> KEKTGQVKHKNQATHKEFSQLEKKFDARLGVYAIDTGTNQTIAYRPNE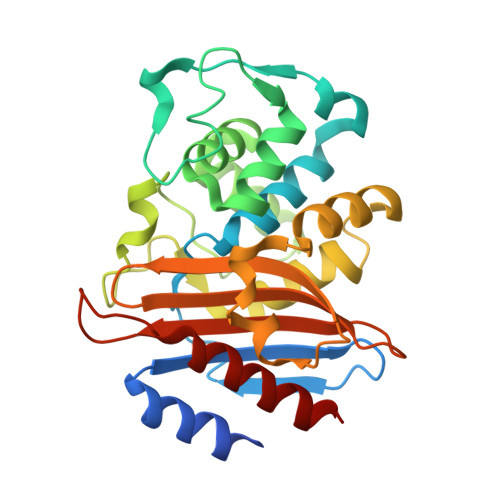RFAFASTYKALAAGVLLQQNSTKKLDEVITYTKEDLVDYSPVTEKHVDTGMTLGEIAEAAVRYSDNTAGNILFHKIGGPKGYEKALRQMGDRVTMSDRFETELNEAIPGDIRDTSTAKAIATNLKAFTAGNALPNHKRNILTKWMKGNATGDKLIRAGVPTNWVVADKSGAGSYGTRNDIAIVWPPNRAPIIIAILSSKDEKGATYDNQLIAEAAEVIVNAFR>[5x]MTDMNILDLFLKASLLVKLIMLILIGFSIASWAIIIQRTRILNAAAREAEAFEDKFWSGIELSRLYQESQGKRDNLTGSEQIFYSGFKEFVRLHRANSHAPEAVVEGASRAMRISMNRELENLETHIPFLGTVGSISPYIGLFGTVWGIMHAFIALGAVKQATLQMVAPGIAEALIATAIGLFAAIPAVMAYNRLNQRVNKLELNYDNFMEEFTAILHRQAFTVSESNKG;>[2x]MARARGRGRRDLKSEINIVPLLDVLLVLLLIFMATAPIITQSVEVDLPDATESQAVSSNDNPPVIVEVSGIGQYTVVVEKDRLERLPPEQVVAEVSSRFKANPKTVFLIGGAKDVPYDEIIKALNLLHSAGVKSVGLMTQPILEHHHHHHHH;> MSKATEQNDKLKRAIIISAVLHVILFAALIWSSFDENIEASAGGGGGSSIDAVMVDSGAVV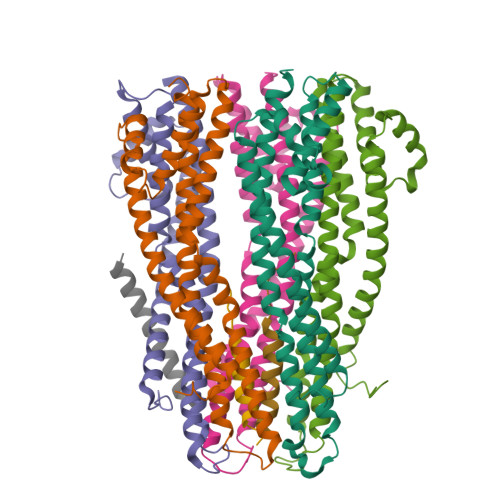EQYKRMQSQESSAKRSDEQRKMKEQQAAEELREKQAAEQERLKQLEKERLAAQEQKKQAEEAAKQAELKQKQAEEAAAKAAADAKAKAEADAKAAEEAAKKAAADAKKKAEAEAAKAAAEAQKKAEAAAAALKKKAEAAEAAAAEARKKAATEAAEKAKAEAEKKAAAEKAAADKKAAAEKAAADKKAAEKAAAEKAAADKKAAAEKAAADKKAAAAKAAAEKAAAAKAAAEADDIFGELSSGKNAPKTGGGAKGNNASPAGSGNTKNNGASGADINNYAGQIKSAIESKFYDASSYAGKTCTLRIKLAPDGMLLDIKPEGGDPALCQAALAAAKLAKIPKPPSQAVYEVFKNAPLDFKP methyl 9-[(2-fluoranyl-4-methoxy-phenyl)amino]-[1,3]thiazolo[5,4-f]quinazoline-2-carboximidate | 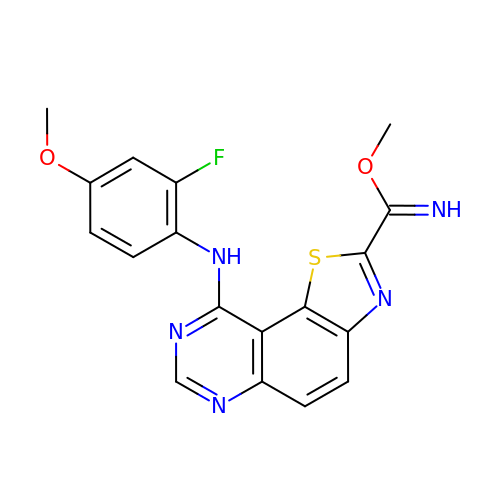C18 H14 F N5 O2 S | RYBNARZBIXTFJS-CAPFRKAQSA-N>[2x]GNSDDARTSIEQRSNAVSQVLLGIFSYVRWPKEPAVLQLCVVGPTEYADGLLRGMVQANGRRVHAERRAVDNPDLGTLCNVIYLGVVDERERQQVFRSLAGHPVLSISERGTECSVGSMFCLNVGGPRITFEANLDSIARSGVRVHPSVLKLARRQATP;>[2x]GLSAEQIAVPQEQGFELRDEGWEFGMSSKVLFGNNLDRLNPDSRNTLTKIARALLAVDIDKVRLEGHTDNYGDEGYNQKLSERRAESVAAVFREAGMPAANIEVRGLGMSKPVADNKTRAGRSENRRVAIIVPAE

The YfiBNR system contains three protein members and modulates intracellular c-di-GMP levels in response to signals received in the periplasm. YfiN is repressed by specific interaction between its periplasmic PAS domain and the periplasmic protein YfiR. YfiB is an OmpA/Pal-like outer-membrane lipoprotein that can activate YfiN by sequestering YfiR in an unknown manner. Previous studies suggested that in response to cell stress, YfiB in the outer membrane sequesters the periplasmic protein YfiR, releasing its inhibition of YfiN on the inner membrane and thus inducing the diguanylate cyclase activity of YfiN to allow c-di-GMP production.

As expected, both mutants form a stable complex with YfiR. Finally, we crystalized YfiR in complex with the YfiBL43P mutant and solved the structure at 1.78 Å resolution by molecular replacement using YfiR and YfiB as models. The YfiB-YfiR complex is a 2:2 heterotetramer in which the YfiR dimer is clamped by two separated YfiBL43P molecules with a total buried surface area of 3161.2 Å2. The YfiR dimer in the complex is identical to the non-oxidized YfiR dimer alone, with only Cys145-Cys152 of the two disulfide bonds well formed, suggesting Cys71-Cys110 disulfide bond formation is not essential for forming YfiB-YfiR complex. The N-terminal structural conformation of YfiBL43P, from the foremost N-terminus to residue D70, is significantly altered compared with that of the apo YfiB. The majority of the α1 helix (residues 34–43) is invisible on the electron density map, and the α2 helix and β1 and β2 strands are rearranged to form a long loop containing two short α-helix turns, thus embracing the YfiR dimer. The YfiB-YfiR interface can be divided into two regions. Region I is formed by numerous main-chain and side-chain hydrophilic interactions between residues E45, G47 and E53 from the N-terminal extended loop of YfiB and residues S57, R60, A89 and H177 from YfiR (Fig. 3D-I(i)). In region II, the side chains of R96, E98 and E157 from YfiB interact with the side chains of E163, S146 and R171 from YfiR, respectively. In the YfiB-YfiR complex, one sulfate ion is found at the bottom of each YfiBL43P molecule and forms a strong hydrogen bond with D102 of YfiBL43P. Similarly, in the YfiR-bound YfiBL43P structure, the sulfate ion interacts with the side-chain atoms of D102 (corresponding to D71 in Pal) and R117 (corresponding to R86 in Pal) and the main-chain amide of N68 (corresponding to D37 in Pal).>[6x]TDTTNSIKHVISPLARQTLQDRDLTRPVAGKRPIRLLPWLQVVKIGGRVMDRGADAILPLVEELRKLLPEHRLLILTGAGVRARHVFSVGLDLGLPVGSLAPLAASEAGQNGHILAAMLASEGVSYVEHPTVADQLAIHLSATRAVVGSAFPPYHHHEFPGSRIPPHRADTGAFLLADAFGAAGLTIVENVDGIYTADPNGPDRGQARFLPETSATDLAKSEGPLPVDRALLDVMATARHIERVQVVNGLVPGRLTAALRGEHVGTLIRTGVRPA;>[6x]ANSTAELEELLMQRSLTDPQLQAAAAAAADFRILPDATVIKIGGQSVIDRGRAAVYPLVDEIVAARKNHKLLIGTGAGTRARHLYSIAAGLGLPAGVLAQLGSSVADQNAAMLGQLLAKHGIPVVGGAGLSAVPLSLAEVNAVVFSGMPPYKLWMRPAAEGVIPPYRTDAGCFLLAEQFGCKQMIFVKDEDGLYTANPKTSKDATFIPRISVDEM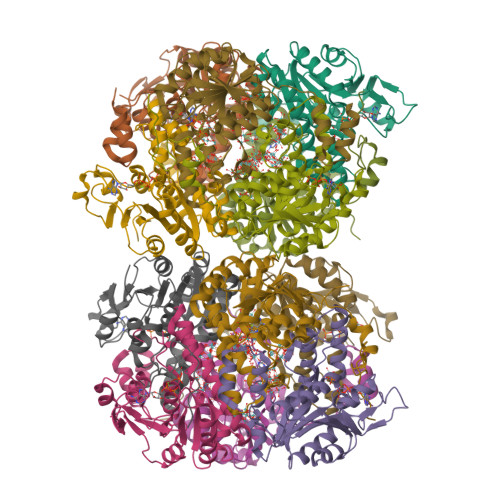KAKGLHDSILEFPVLDLLQSAQHVREVQVVNGLVPGNLTRALAGEHVGTIITAS> NRFYLLTLTSNQDESITLAIDVEDMVAVAYQPAGSHESYFFLNAPQIAFHTLFTDTHQNVLNFDNTFKSLENAAGTTRQ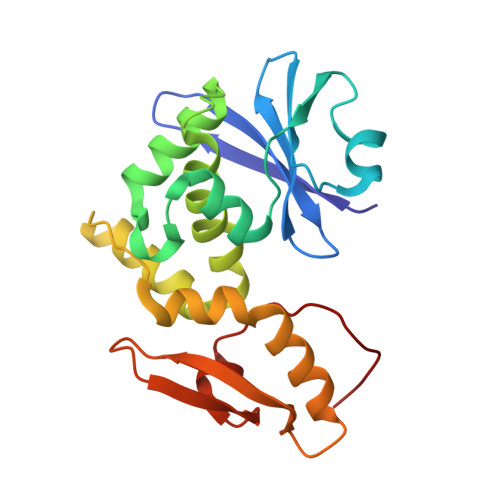TIVLGVDPLDFAISNLFNADPKLLPLSFLVIIQMVLEASKFRFIEQSVAYSFKNEKTFLPDLAIVSLEDNWSEISLQIQASTSLQGLFGSVVELYNSNNELIEVDSIYYPIILANVALQLYHCQVST N-[3-(1H-pyrazol-3-yl)phenyl]-1H-indazole-7-carboxamide | C17 H13 N5 O | 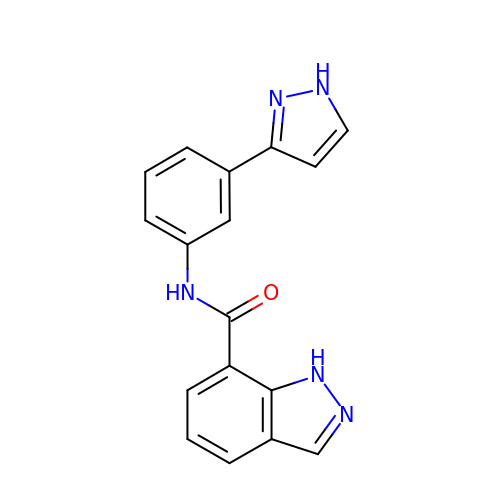HELOGTPQLUDSEC-UHFFFAOYSA-N>MNLKNLIIYEAFARAYPGEKGKKFLSLEKDLERLKGMGINTVWLMPIHPTGVEGRKGTLGSPYAIRDYYEIDLLIGTKGDFKKFVKRAHELNMYVLMDMVLNHAAVDNVLVKKHPEWFLRDENGNPTRKVPDWSDVVDFDYSNGELREYMINMMRYWVEEFDVDGFRCDVAGLVPLDFWLQARKNLDPVKRLIWISETHDPYMYQAFDITYDYDGYYRFRDFIEGKNSLREYIDFLRMQDHMYPRGYIKMRFLENHDQPRVAKFLSRESLMHWIAFLFTVKGVPLVHNGQEYALKEDLDIFNEYTLPIPGEENEIFSLHRKLAHYRYKTNVFSNGEMIFIRNDQPE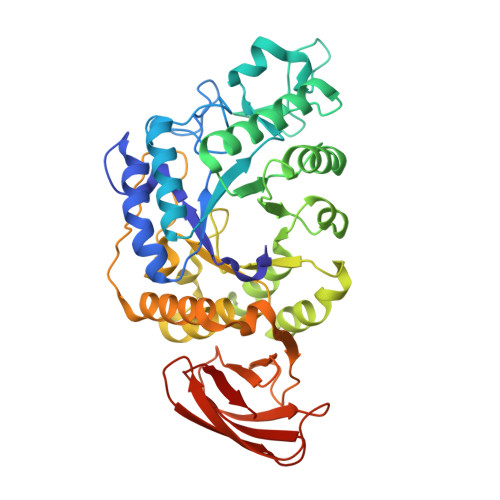RVISYLWRHGNRFILCVLNPLLENTSVTLDFSGIWENICIHSKNVFNDDIVRVSVKNSRAKIKVGREPLILSFVLY[2x]>MAKKTSSKGKLPPGPSPLPVLGNLLQMDRKGLLRSFLRLREKYGDVFTVYLGSRPVVVLCGTDAIREALVDQAEAFSGRGKIAVVDPIFQGYGVIFANGERWRALRRFSLATMRDFGMGKRSVEERIQEEARCLVEELRKSKGALLDNTLLFHSITSNIICSIVFGKRFDYKDPVFLRLLDLFFQSFSLISSFSSQVFELFSGFLKYFPGTHRQIYRNLQEINTFIGQSVEKHRATLDPSNPRDFIDVYLLRMEKDKSDPSSEFHHQNLILTVLSLFFAGTETTSTTLRYGFLLMLKYPHVTERVQKEIEQVIGSHRPPALDDRAKMPYTDAVIHEIQRLGDLIPFGVPHTVTKDTQFRGYVIPKNTEVFPVLSSALHDPRYFETPNTFNPGHFLDANGALKRN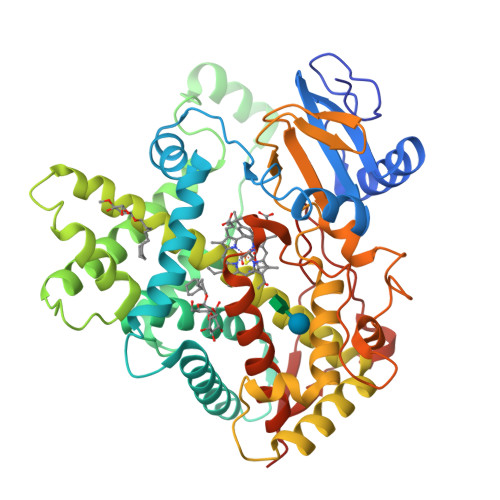EGFMPFSLGKRICLGEGIARTELFLFFTTILQNFSIASPVPPEDIDLTPRESGVGNVPPSYQIRFLARHHHH[4x]>MSTGGDFGNPLRKFKLVFLGEQSVGKTSLITRFMYDSFDNTYQATIGIDFLSKTMYLEDRTIRLQLWDTAGLERFRSLIPSYIRDSAAAVVVYDITNVNSFQQTTKWIDDVRTERGSDVIIMLVGNKTDLADKRQVSIEEGERKAKELNVMFIETSAKAGYNVKQLFRRVAAALPGMESTQDRSR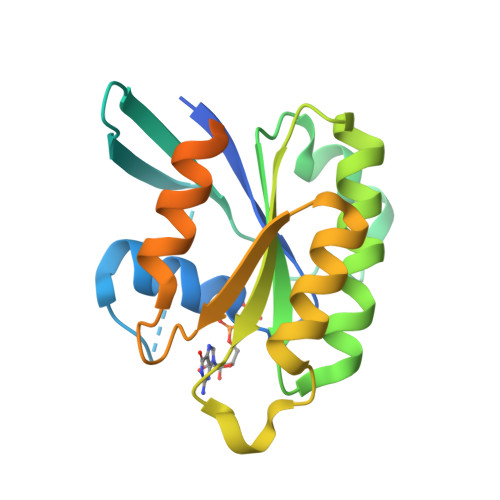EDMIDIKLEKPQEQPVSEGGCSCLEHHHHHH[2x]> MKIKD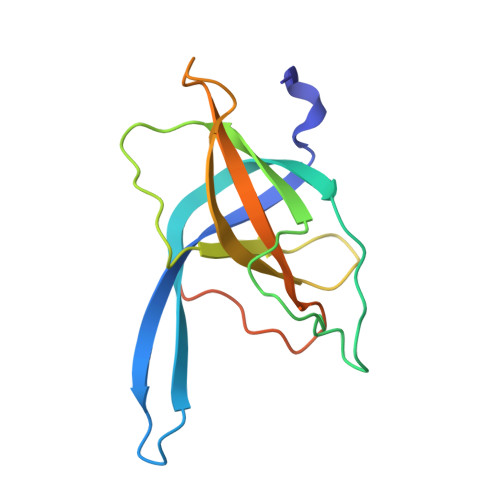RKHRVIVCSQKSDVDDNGQLLISRTGSINGWAAIEPVKAIRFSKDGVSMQKDTFQPTHDITMNYNPDVNISVSAWVYEHRLKSPPRWFKVISVINVDECSQFMRLRSRLVESNDEVEKPVSEENSFGAVKIDIPL> PISPIETVPVKLKPGMDGPKVKQWPLTEEKIKALVEICTEMEKEGKISKIGPENPYNTPVFAIKKKDSTKWRKLVDFRELNKRTQDFWEVQLGIPHPAGLKKKKSATVLDVGDAYFSVPLDEDFRKYTAFTIPSINNETPGIRYQYNVLPQGWKGSPAIFQSSMTKILEPFRKQNPDIVICQYMDDLYVGSDLEIGQHRTKIEELRQHLLRWGLTTPDKKHQKEPPFLWMGYELHPDKWTVQPIVLPEKDSWTVNDIQKLVGKLNWASQIYPGIKVRQLCKLLRGTKALTEVIPLTEEAELELAENREILKEPVHGVYYDPSKDLIAEIQKQGQGQWTYQIYQEPFKNLKTGKYARMRGAHTNDVKQLTEAVQKITTESIVIWGKTPKFKLPIQKETWETWWTEYWQATWIPEWEFVNTPPLVKLWYQLEKEPIVGAETFYVDGAANRETKLGKAGYVTNRGRQKVVTLTDTTNQKTELQAIYLALQDSGLEVNIVTDSQYALGIIQAQPDQSESELVNQIIEQLIKKEKVYLAWVPAHKGIGGNEQVDKLVSAGIRKVL;> PISPIETVPVKLKPGMDGPKVKQWPLTEEKIKALVEICTEMEKEGKISKIGPENPYNTPVFAIKKKDSTKWRK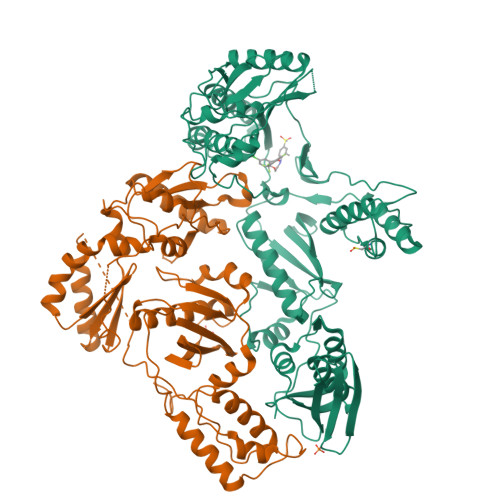LVDFRELNKRTQDFWEVQLGIPHPAGLKKKKSATVLDVGDAYFSVPLDEDFRKYTAFTIPSINNETPGIRYQYNVLPQGWKGSPAIFQSSMTKILEPFRKQNPDIVICQYMDDLYVGSDLEIGQHRTKIEELRQHLLRWGLTTPDKKHQKEPPFLWMGYELHPDKWTVQPIVLPEKDSWTVNDIQKLVGKLNWASQIYPGIKVRQLCKLLRGTKALTEVIPLTEEAELELAENREILKEPVHGVYYDPSKDLIAEIQKQGQGQWTYQIYQEPFKNLKTGKYARMRGAHTNDVKQLTEAVQKITTESIVIWGKTPKFKLPIQKETWETWWTEYWQATWIPEWEFVNTPPLVKLWYQLEKEPIVGAETF>[6x]GSHVSKREDGRLDHELRPVIITRGFTENPAGSVLIEFGHTKVLCTASVTEGVPRWRKATGLGWLTAEYAMLPSATHSRSDRESVRGRLSGRTQEISRLIGRSLRACIDLAALGENTIAIDCDVLQADGGTRTAAITGAYVALADAVTYLSAAGKLSDPRPLSCAIAAVSVGVVDGRIRVDLPYEEDSRAEVDMNVVATDTGTLVEIQGTGEGATFARSTLDKLLDMA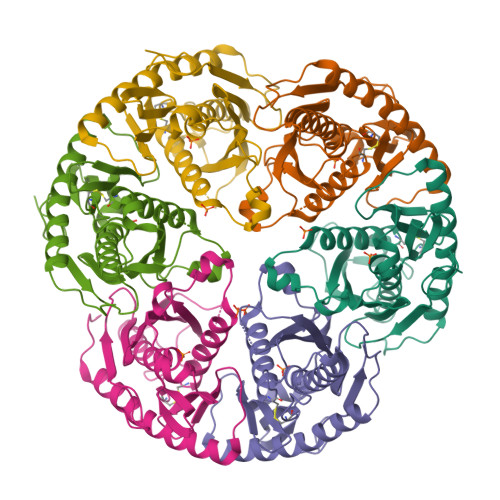LGACDTLFAAQRDALALPYPGVLPQGPPPPKAFGT> MDKFCNSTFWDLSLLESPEADLPLCFEQTVLVWIPLGFLWLLAPWQLYSVYRSRTKRSSITKFYLAKQVFVVFLLILAAIDLSLALTEDTGQATVPPVRYTNPILYLCTWLLVLAVQHSRQWCVRKNSWFLSLFWILSVLCGVFQFQTLIRALLKDSKSNMAYSYLFFVSYGFQIVLLILTAFSGPSDSTQTPSVTASFLSSITFSWYDRTVLKGYKHPLTLEDVWDIDEGFKTRSVTSKFEAAMTKDLQKARQAFQRRLQKSQRKPEATLHGLNKKQSQSQDVLVLEEAKKKSEKTTKDYPKSWLIKSLFKTFHVVILKSFILKLIHDLLVFLNPQLLKLLIGFVKSSNSYVWFGYICAILMFAVTLIQSFCLQSYFQHCFVLGMCVRTTVMSSIYKKALTLSNLARKQYTIGETVNLMSVDSQKLMDATNYMQLVWSSVIQITLSIFFLWRELGPSILAGVGVMVLLIPVNGVLATKIRNIQVQNMKNKDKRLKIMNEILSGIKILKYFAWEPSFQEQVQGIRKKELKNLLRFGQLQSLLIFILQITPILVSVVTFSVYVLVDSANVLNAEKAFTSITLFNILRFPLSMLPMVTSSILQASVSVDRLERYLGGDDLDTSAIRRVSNFDKAVKFSEASFTWDPDLEATIQDVNLDIKPGQLVAVVGTVGSGKSSLVSAMLGEMENVHGHITIQGSTAYVPQQSWIQNGTIKDNILFGSEYNEKKYQQVLKACALLPDLEILPGGDMAEIGEKGINLSGGQKQRVSLARAAYQDADIYILDDPLSAVDAHVGKHIFNKVVGPNGLLAGKTRIFVTHGIHFLPQVDEIVVLGKGTILEKGSYRDLLDKKGVFARNWKTFMKHSGPEGEATVNNDSEAEDDDDGLIPTMEEIPEDAASLAMRRENSLRRTLSRSSRSSSRRGKSLKNSLKIKNVNVLKEKEKEVEGQKLIKKEFVETGKVKFSIYLKYLQAVGWWSILFIILFYGLNNVAFIGSNLWLSAWTSDSDNLNGTNNSSSHRDMRIGVFGALGLAQGICLLISTLWSIYACRNASKALHGQLLTNILRAPMRFFDTTPTGRIVNRFSGDISTVDDLLPQTLRSWMMCFFGIAGTLVMICMATPVFAIIIIPLSILYISVQVFYVATSRQLRRLDSVTKSPIYSHFSETVTGLPIIRAFEHQQRFLAWNEKQIDINQKCVFSWITSNRWLAIRLELVGNLVVFCSALLLVIYRKTLTGDVVGFVLSNALNITQTLNWLVRMTSEAETNIVAVERISEYINVENEAPWVTDKRPPADWPRHGEIQFNNYQVRYRPELDLVLKGITCNIKSGEKVGVVGRTGAGKSSLTNCLFRILESAGGQIIIDGIDVASIGLHDLRERLTIIPQDPILFSGSLRMNLDPFNKYSDEEVWRALELAHLRSFVSGLQLGLLSEVTEGGDNLSIGQRQLLCLGRAVLRKSKILVLDEATAAVDLETDSLIQTTIRKEFSQCTVITIAHRLHTIMDSDKIMVLDNGKI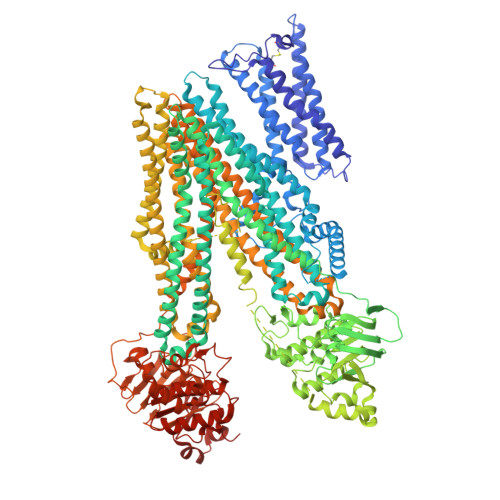VEYGSPEELLSNRGSFYLMAKEAGIENVNHTEL>LKESPSGYLRSGEGDTGCGELVWVGEPLTLRTAETITGKYGVWMRDPKPTYPYTQETTWRIDTVGTDVRQVFEYDLISQFMQGYPSKVHILPRPLESTGAVVYSGSLYFQGAESRTVIRYELNTETVKAEKEIPGAGYHGQFPYSWGGYTDIDLAVDEAGLWVIYSTDEAKGAIVLSKLNPENLELEQTWETNIRKQSVAEAFIICGTLYTVSSYTSADATVNFAYDTGTGISKTLTIPFKNRYKYSSMISYNPLEKKLFAWDNLNMVTYDIKLSKM[2x]

Olfactomedins (OLFs), modular proteins containing an OLF domain that are predominantly expressed in neural tissues, are involved in fundamental processes of cell growth, cell signaling and cell adhesion. High-resolution crystal structures of the ∼30 kDa five-bladed β-propeller OLF domain are available for four subfamily members: olfactomedin-1, latrophilin, myocilin and gliomedin. While the folds are nearly indistinguishable [Fig. 1(a)], one difference is the presence or absence of a heptacoordinate calcium ion bound in the central internal solvent-filled cavity of the β-propeller [Fig. 1(b)]. To survey the OLF triads for calcium binding and to test whether calcium binding can be reverted by simultaneously altering Asn428 to an acidic Asp or Glu, we replaced the triad Asp–Asn–Asp with Asp–Glu–Ser, Asp–Asp–His and Asp–Glu–Lys via site-directed mutagenesis of Asn428 and Asp478.

Asp–Glu–Ser is the second-ranked triad in Arthropoda. In the case of myoc-OLFN428E/D478S the conversion of Asn428 to Glu decreases the stability compared with the previously characterized myoc-OLFD478S, reverting to the value for myoc-OLFWT. For myoc-OLFN428D/D478H, nearly all residues were traced; residues 291–292 in monomer A and residues 292–293 in monomer B could not be traced, although several loops in both molecules were difficult to model, suggesting overall loop flexibility for this variant as well. Among the well ordered loops is one encompassing residues 259–268, which is shifted ∼5 Å in myoc-OLFN428D/D478H and myoc-OLFN428E/D478S compared with the analogous residues forming the top helical turn in myoc-OLFWT [top and middle in Figs. 3(a) and 3(c)]. Given the strong (for myoc-OLFN428E/D478S) and marginal (myoc-OLFN428D/D478H) stabilization by Ca2+ seen by DSF, we considered assigning either of these difference peaks as a Ca2+, but were ultimately unable to confirm calcium in either variant. Calcium coordination for the more likely variant myoc-OLFN428E/D478S was not readily satisfied by the available protein ligands or water (not shown). To support the absence of Ca2+ in the structure, we employed a strategy used recently to identify Ca2+ ions by anomalous scattering. Our data only reveal anomalous difference peaks from sulfur [Cys245–Cys435 disulfide (not shown) and selected methionines; Supplementary Fig S4(a)]. In sum, unlike myoc-OLFWT, neither myoc-OLFN428D/D478H nor myoc-OLFN428E/D478S copurifies with a fully occupied Ca2+, but both the Nematoda triad Asp–Asp–His and the Arthropoda triad Asp–Glu–Ser appear to be able to support metal-ion binding, perhaps in certain bio­logical contexts.(2R,4S)-2-[(1S)-1-({[3-(2-chlorophenyl)-5-methyl-1,2-oxazol-4-yl]carbonyl}amino)-2-oxoethyl]-5,5-dimethyl-1,3-thiazolidine-4-carboxylic 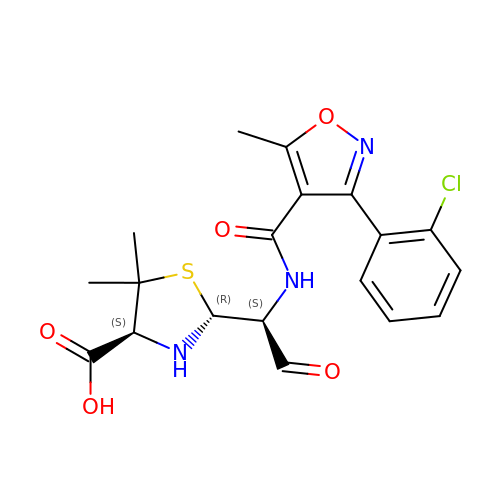acid | C19 H20 Cl N3 O5 S | DMRXQBXKFQMOBD-YLQAJVPDSA-N>PSVYDAAAQLTADVKKDLRDSWKVIGSDKKGNGVALFTTLFADNQETIGYFKRLGDVSQGMANDKLRGHSITLMYALQNFIDQLDNPDDLVCVVEKFAVNHITRKISAAEFGKINGPIKKVLASKNFGDK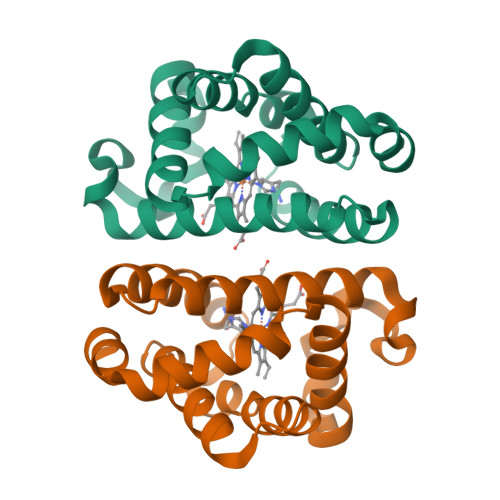YANAWAKLVAVVQAAL[2x]> KK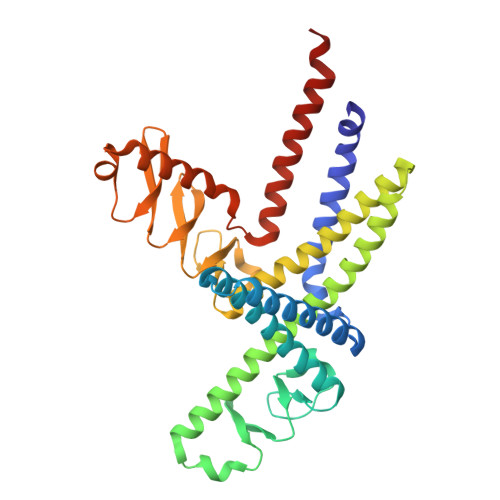LDKLERQGKDLEDKYKTYEENLEGFEKLLTDSEELSLSEINEKMKAFSKDSEKLTQLMEKHKGDEKTVQSLQREHHDIKAKLANLQVLHDAHTGKKSYVNEKGNPVSSLKDAHLAINKDQEVVEHKGQFYLLQKGQWDAIKNDPAALEKAQKDYSQSKHDLATIKMEALIHKLSLEMEKQLETINDLIMSTDPKENEEATKLLHKHNGLNLKLANLQDMLAVHRKEKSFFNEKGEKVTSLNDAHYVIGKDQQLFNLGGKFYPIHKEQKILEKDGKFYLLKQGEDWESIKDSPEKQKKAEHDFHKLQYETPMTVKKLVHHNKGLETTIHKERIEELEHHHHHH>QVTPRPEAAPGARPGFRAPARIISPEIMPDNKVTFRVYSKDASKVTITGEWQTGPGGVEELVKNDTGMFSITVGPLKPELYAYNFTVDGVKALDANNVQVRRDGTNYQNFFIIPGPESDLYFHKNNVPHGTVTKVWYKSSVIGFDRRMYVYTPAGYEGDTQRYPVFYLLHGAGGDEDAWTNMGRTAQIMDNLIAQGKAKPMIVVMTNGNANQAGAQNEVPPVPVTQGQQGIPSGSGMTGKFEEHLVKDVVPFIEKNFRAL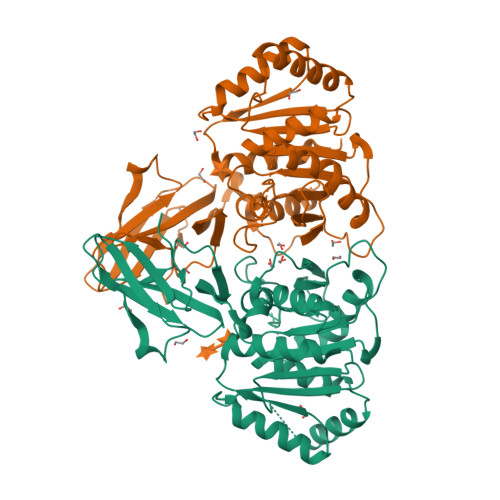TGKDNRAIAGLSMGGGHTQTITNDNPGMFSYIGVFSMGIMAGRQQGADAEKIEKERDAKIEALKKSGYKLYWIACGKDDFVYQSALTLRNTLDKHNFKYVYRESTGGHTWANWRIYLSEFAPMLFKLL[2x]>MIPLLAFAAWSGTGKTTLLKKLIPALCARGIRPGLIKHTHHDMDVDKPGKDSYELRKAGAAQTIVASQQRWALMTETPDEEELDLQFLASRMDTSKLDLILVEGFKHEEIAKIVLFRDGAGHRP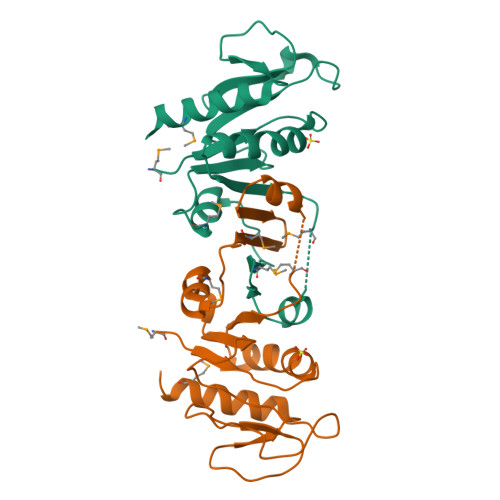EELVIDRHVIAVASDVPLNLDVALLDINDVEGLADFVVEWMQKQNG[2x]>[2x]GRSRLLEDFRNNRYPNLQLREIAGHIMEFSQDQHGSRFIQLKLERATPAERQLVFNEILQAAYQLMVDVFGNYVIQKFFEFGSLEQKLALAERIRGHVLSLALQMYGCRVIQKALEFIPSDQQNEMVRELDGHV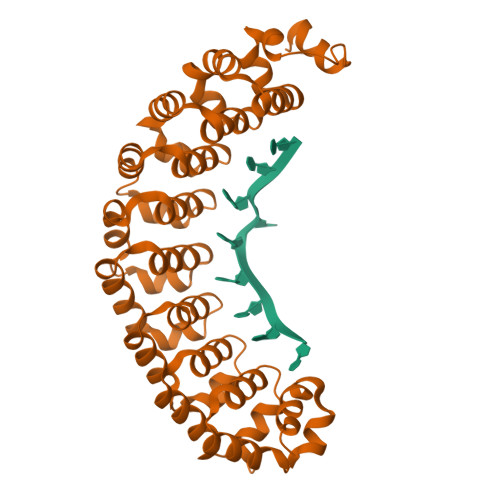LKCVKDQNGNHVVQKCIECVQPQSLQFIIDAFKGQVFALSTHPYGCRVIQRILEHCLPDQTLPILEELHQHTEQLVQDQYGNYVIQHVLEHGRPEDKSKIVAEIRGNVLVLSQHKFASNVVEKCVTHASRTERAVLIDEVCTMNDGPHSALYTMMKDQYANYVVQKMIDVAEPGQRKIVMHKIRPHIATLRKYTYGKHILAKLEKYYMK(2~{S})-2-[[(2~{R})-4-methyl-1-oxidanyl-1-oxidanylidene-pentan-2-yl]carbamoyloxy]pentanedioic acid | C12 H19 N O8 | 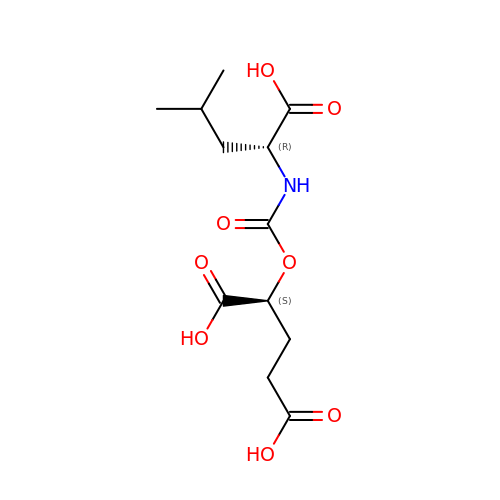WQDZXAWSGIQGKR-SFYZADRCSA-N>[2x]MATATEQWVLVEMVQALYEAPAYHLILEGILILWIIRLLFSKTYKLQERSDLTVKEKEELIEEWQPEPLVPPVPKDHPALNYNIVSGPPSHKTVVNGKECINFASFNFLGLLDNPRVKAAALASLKKYGVGTCGPRGFYGTFDVHLDLEDRLAKFMKTEEAIIYSYGFATIASAIPAYSKRGDIVFVDRAACFAIQKGLQASRSDIKLFKHNDMADLERLLKEQEIEDQKNPRKARVTRRFIVVEGLYMNTGTICPLPELVKLKYKYKARIFLEESLSFGVLGEHGRGVTEHYGINIDDIDLISANMENALASIGGFCCGRSFVIDHQRLSGQGYCFSASLPPLLAAAAIEALNIMEENPGIFAVLKEKCGQIHKALQGISGLKVVGESLSPAFHLQLEESTGSREQDVRLLQEIVDQCMNRSIALTQARYLEKEEKCLPPPSIRVVVTVEQTEEELERAASTIKEVAQAVLL;>[2x]MRPEPGGCCCRRTVRANGCVANGEVRNGYVRSSAAAAAAAAAGQIHHVTQNGGLYKRPFNEAFEETPMLVAVLTYVGYGVLTLFGYLRDFLRYWRIEKCHHATEREEQKDFVSLYQDFENFYTRNLYMRIRDNWNRPICSVPGARVDIMERQSHDYNWSFKYTGNIIKGVINMGSYNYLGFARNTGSCQEAAAKVLEEYGAGVCSTRQEIGNLDKHEELEELVARFLGVEAAMAYGMGFATNSMNIPALVGKGCLILSDELNHASLVLGARLSGATIRIFKHNNMQS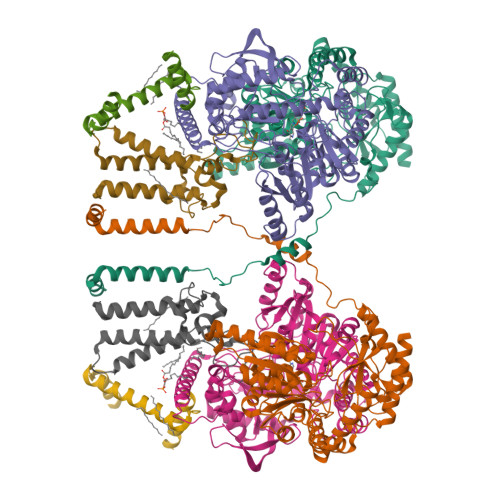LEKLLKDAIVYGQPRTRRPWKKILILVEGIYSMEGSIVRLPEVIALKKKYKAYLYLDEAHSIGALGPTGRGVVEYFGLDPEDVDVMMGTFTKSFGASGGYIGGKKELIDYLRTHSHSAVYATSLSPPVVEQIITSMKCIMGQDGTSLGKECVQQLAENTRYFRRRLKEMGFIIYGNEDSPVVPLMLYMPAKIGAFGREMLKRNIGVVVVGFPATPIIESRARFCLSAAHTKEILDTALKEIDEVGDLLQLKYSRHRL;>[2x]MAGMALARAWKQMSWFYYQYLLVTALYMLEPWERTVFNSMLVSIVGMALYTGYVFMPQHIMAILHYFEIVQ;>[2x]MNVGTAHSEVNPNTRVMNSRGIWLSYVLAIGLLHIVLLSIPFVSVPVVWTLTNLIHNMGMYIFLHTVKGTPFETPDQGKARLLTHWEQMDYGVQFTASRKFLTITPIVLYFLTSFYTKYDQIHFVLNTVSLMSVLIPKLPQLHGVRIFGINKY> FSELLDLVGGLGRFQVLQTMALMVSIMWLCTQSMLENFSAAVPSHRCWAPLLDNSTAVSTSLSPEALLAISIPPGPNQRPHQCRRFRQPQWQLLDPNATATSWSEADTEPCVDGWVYDRSIFTSTIVAKWNLVCDSHALKPMAQSIYLAGILVGAAACGPASDRFGRRLVLTWSYLQMAVMGTAAAFAPAFPVYCLFRFLLAFAVAGVMMNTGTLLMEWTAARARPLVMTLNSLGFSFGHGLTAAVAYGVRDWTLLQLVVSVPFFLCFLYSWWLPESARWLIIKGKPDQALQELRKVARINGHKEAKNLTIEVLMSSVKEEVASAKEPRSVLDLFCVPGLRFRTCISTLCWFAFGFTFFGLALDLQALGSNIFLLQMFIGVVDIPAKMGALLLLSHLGRRPTLAASLLLAGLCILANTLVPHEMGALRSALAVLGLGGVGAAFTCITIYSSELFPTVLRMTAVGLGQMAARGGAILGPLVRLLGVHGPWLPLLVYGTVPVLSGLAALLLPETQSLPLPDTIQDVQNQAVKKATHGTLGNSVLKSTQF

Among the several renal transporters involved in urate flux, urate transporter 1 (URAT1) is the primary one responsible for urate reabsorption. URAT1, or SLC22A12, belongs to the organic anion transporter (OAT) subgroup of the solute carrier family 22 (SLC22).6,13 It functions as an antiporter, moving intracellular organic anions or chloride ions to drive the uptake of extracellular urate from the renal tubule lumen into the cells. URAT1 is also an established therapeutic target for the treatment of hyperuricemia and gout. URAT1 adopts a canonical major facilitator superfamily fold, with twelve transmembrane helices (TMs).

In the presence of urate, we captured URAT1 in multiple conformations that represent major states in the transport cycle: outward-facing (cavity open to the extracellular side), occluded (cavity inaccessible to either side), and inward-facing. In all three conformations, urate binds to a similar location in the central cavity and this binding mode is notably different from previous predictions by molecular docking on homology models of URAT1.34,35 In our structures, the urate binding site is surrounded by several bulky aromatic residues, with five phenylalanines (Phe241, Phe360, Phe364, Phe365, and Phe449) forming a hydrophobic cage that encapsulates urate with hydrophobic and π–π stacking interactions. Urate binding to the outward-facing conformation induces the closure of the extracellular gate in TM1 and TM7, leading to occlusion of the central cavity by Met36, Asn39, Leu369 and Leu371. We observed that as the transporter transitions from the outward-facing to the occluded conformations, the side chain of Arg477 swings away from the pocket, weakening its interaction with urate (left to middle). The transitions from outward-facing to occluded to inward-facing conformations also include the opening of the intracellular gate. The intracellular gate begins to loosen in the occluded state and fully opens in the inward-facing state, permitting urate release into the cell.(2S,4S)-1-methyl-4-oxidanyl-pyrrolidine-2-carboxylic acid | C6 H11 N O3 | 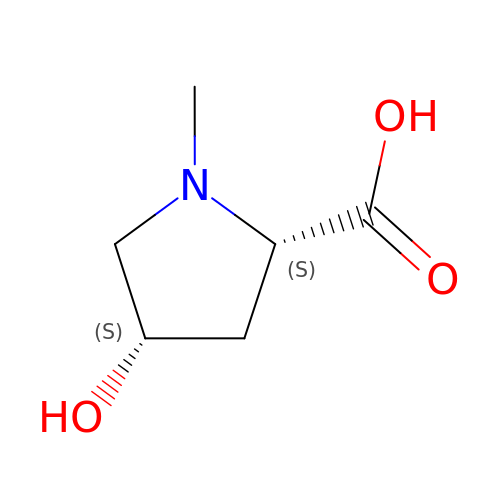FMIPNAUMSPFTHK-WHFBIAKZSA-N>NKNNDKLTLWTTPDTSPNCRIDQDKDSKLTLVLTKCGSQILANVSLIVVAGRYKIINNNTNPALKGFTIKLLFDKNGVLMESSNLGKSYWNFRNQNSIMSTAYEKAIGFMPNLVAYPKPTTGSKKYARDIVYGNIYLGGKPHQPVTIKTTFNQETGCEYSITFDFSWAKTYVNVEFETTSFTFSYIAQE[12x]

Each protein forms key interactions to promote cell infection, with the terminal domain of the fiber, the fiber knob protein, interacting with the viruses’ primary cell entry receptor. The adenovirus fiber knob protein is known to have a highly conserved trimeric structure. Sialic acid (SA) usage has been proposed as a cell infection mechanism for EKC causing HAdV-D. Here we highlight an important role for SA engagement by many HAdV-D. We provide apo state crystal structures of 7 previously undetermined HAdV-D fiber-knob proteins, and structures of HAdV-D25, D29, D30 and D53 fiber-knob proteins in complex with SA. Our findings demonstrate a conserved binding site for sialic acid, common across the species D adenoviruses, therefore suggesting that, along with CAR, the receptor can be used to initiate cell entry.

To evaluate the potential for these recombinant fiber knob proteins to bind cellular sialic acid residues, crystals of the fiber-knob proteins were also soaked with sialic acid prior to data collection. This resulted in four structures of HAdV-D25, D29, D30 and D53 in complex with sialic acid also shown in Fig. 1. Crystals of HAdV-D53 fiber knob protein were too sensitive to soaking, and only very short soaks could rescue any samples suitable for diffraction. The short soak allowed only two of four trimers in the asymmetric unit to bind β-sialic acid, with a significant change in packing, explaining the sensitivity of these crystals to soaking. The conformation of the bound sialic acid was found to be a mixture of the α and β anomers, freely exchangeable in solution and minimal protein side chain adjustment was required to accommodate either conformation. HAdV-D53 is of particular interest due to the recent confirmation of EKC causing infection, similar to previously identified sialic acid binding viruses HAdV-D37 and D64. In contrast, viruses pseudotyped with the fiber-knob protein of HAdV-D26 demonstrated a statistically significant reduction in transduction in all cell lines following cleavage of sialic acid. This was also demonstrated by viruses pseudotyped with an HAdV-D53 fiber knob protein, where all reductions in transduction were also statistically significant in all three cell lines tested. There was an overall trend in reduction, although in BT-20 cells there was a small, non-significant, increase in transduction of HAdV-D29 fiber-knob protein virus following treatment with neuraminidase. These results indicate significant usage of sialic acid by HAdV-D53 fiber-knob proteins, and the potential partial usage across the other species D adenovirus fiber-knob proteins. One of the viruses in this article that demonstrated significantly reduced transduction on removal of sialic acid following neuraminidase treatment is HAdV-D53.7-nitro-2,3-dioxo-2,3-dihydroquinoxaline-6-carbonitrile 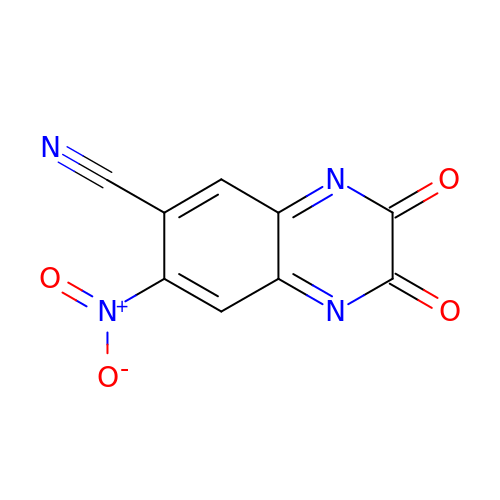| C9 H2 N4 O4 | IAWXTSMHXFRLQR-UHFFFAOYSA-N N-{(1S)-1-[8-chloro-2-(2-methylpyridin-3-yl)quinolin-3-yl]ethyl}-9H-purin-6-amine | C22 H18 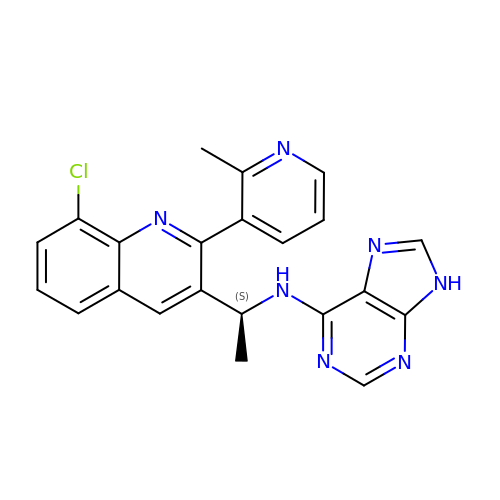Cl N7 | DHDVJIWYMLZLBX-ZDUSSCGKSA-N> MLFFSFFKTLVDQEVVVELKNDIEIKGTLQSVDQFLNLKLDNISCTDEKKYPHLGSVRNIFIRGSTVRYVYLNKNMVDT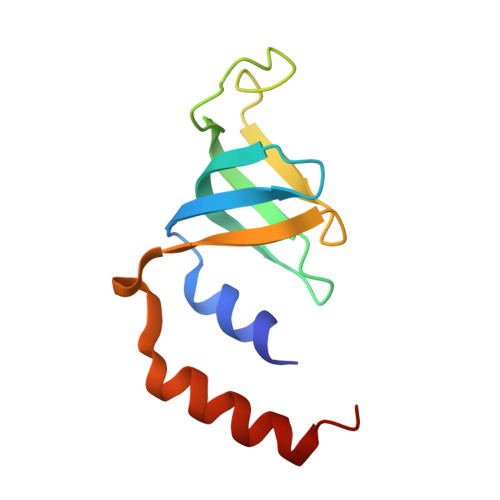NLLQDATRREVMTERK N-[(1R)-4-cyano-2,3-dihydro-1H-inden-1-yl]-4-[(quinazolin-4-yl)amino]benzamide 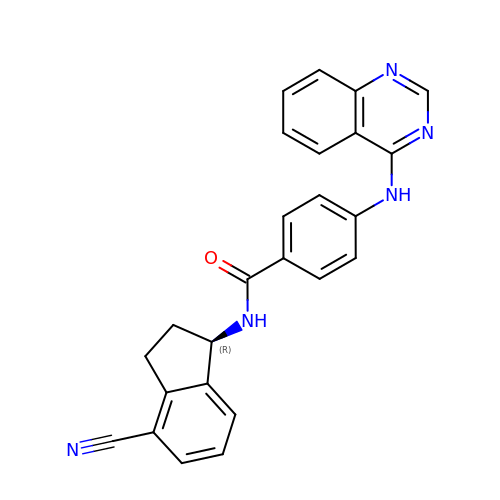| C25 H19 N5 O | PHHSGPIPVMRBMQ-HSZRJFAPSA-N>[2x]SPNYDKWEMERTDITMKH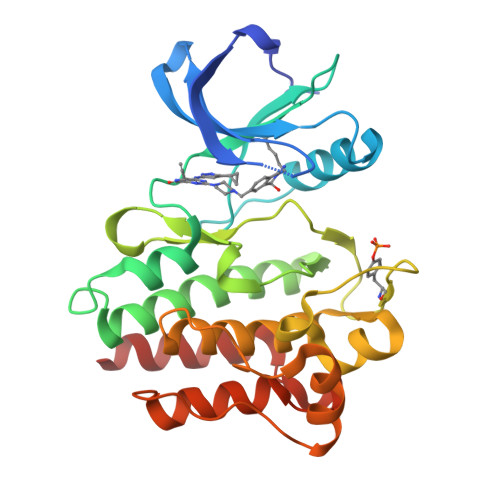KLGGGQKGEVYEGVWKKYSLTVAVXTLKEDTMEVEEFLKEAAVMKEIKHPNLVQLLGVCTREPPFYIITEFMTYGNLLDYLRECNRQEVNAVVLLYMATQISSAMEYLEKKNFIHRDLAARNCLVGENHLVKVADFGLSRLMTGDTYTAHAGAKFPIKWTAPESLAYNKFSIKSDVWAFGVLLWEIATYGMSPYPGIDLSQVYELLEKDYRMERPEGCPEKVYELMRACWQWNPSDRPSFAEIHQAFETMFQES> GSEDLKKLEEEFDVRLGVYAIDTGADKEISYRENERFAYTSTFK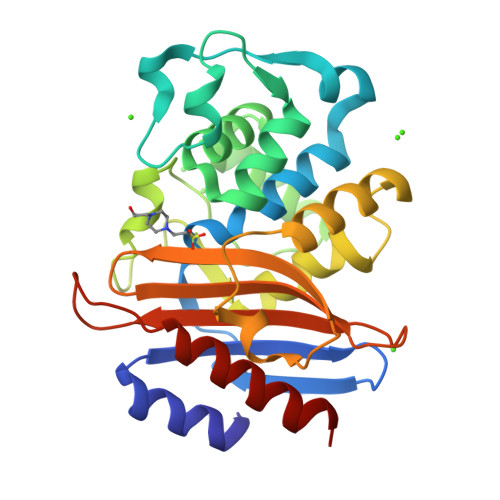PLAVGAVLQTKSDEELEETITYSEEDLVTYSPITEQHVDEGMTLVEIADAAIRYSDNTAGNLLLEAMGGPDELETILRDIGDETIEMDRYETELNEAKPGDIRDTSTAKAMATTLQQYVLEDVLDADRREVLTNMLINNTTGDALIRAGVPDGWTVGDKTGAGGYGTRNDIGIIWPEGDEEPIVIAIMSSRDEEDADYDDKLIEKATEIVLQELRN1-(4-cyanophenyl)-N-(3-fluorophenyl)-3-[4-(methylsulfonyl)phenyl]-1H-pyrazole-4-carboxamide | C24 H17 F N4 O3 S | 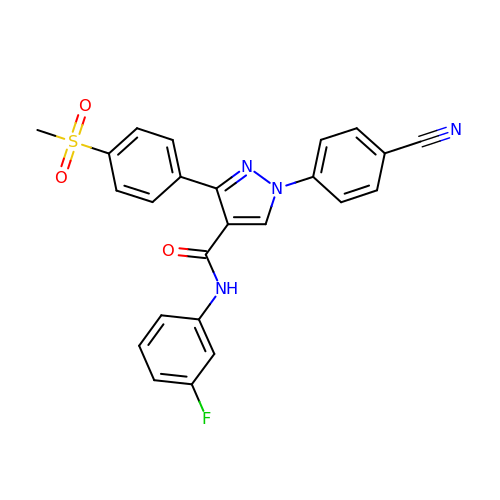ZUWUBCCXJATTTE-UHFFFAOYSA-N> MPETPIMGQDVKYLFQSIDAATGSAPLFPAYQTDGSVSGERELFDEQTKNGRILGPGSVADSGEVTYYGKRGDAGQKAIEDAYQNGKQIKFW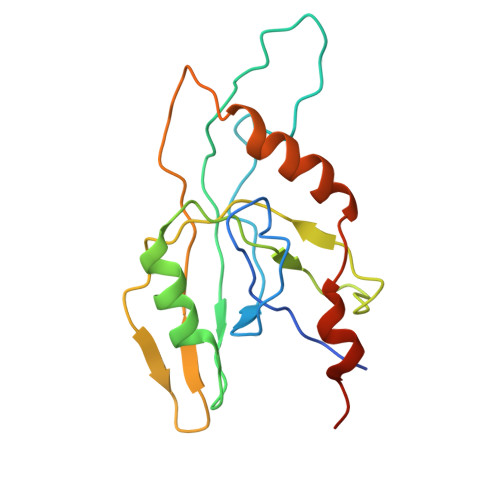RVDTVKNENDKYDAQFGFAYIESREYSDGVEGAVEISISLQVIGELKNGEIDTLPEEIVNVSKGGYDFQQPGQTTGEAPGTVPAP> GPKDNNKTLKPAIAEYIVKKAKQRIALQRWQDELNRRKNHKGMIFVENTVDLEGPPSDFYYINEYKPAPGISLVNEATFGCSCTDCFFQKCCPAEAGVLLAYNKNQQIKIPPGTPIYECNSRCQCGPDCPNRIVQKGTQYSLCIFRTSNGRGWGVKTLVKIKRMSFVMEYVGEV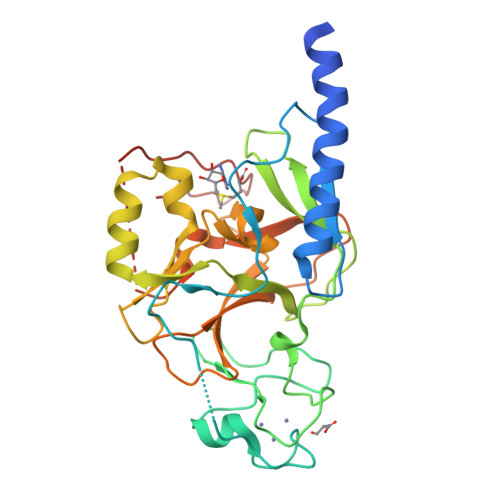ITSEEAERRGQFYDNKGITYLFDLDYESDEFTVDAARYGNVSHFVNHSCDPNLQVFNVFIDNLDTRLPRIALFSTRTINAGEELTFDYQMKGSGDISSDSIDHSPAKKRVRTVCKCGAVTCRGYLN> GEEDLCAAFNVICDNVGKDWRRLARQLKVSDTKIDSIEDRYPRNLTERVRESLRI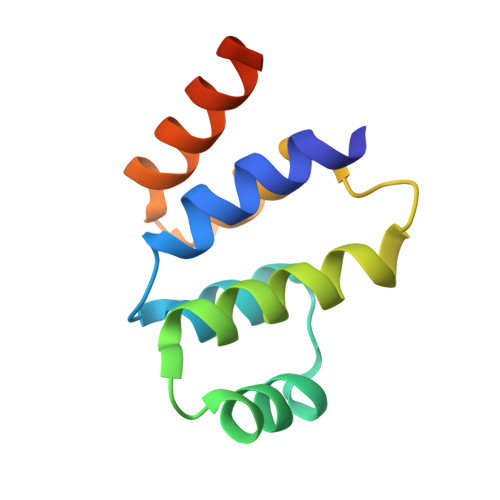WKNTEKENATVAHLVGALRSCQMNLVADLVQEVQQARLEHHHHHH> GDPVEDIIHDALSSTVRRAITSGQDVNTAAGTAPSSHRLETGRVPALQAAETGATSNATDENMIETRCVMNRNGVLEATISHFFSRSGLVGVVNLTDGGTDTTGYAVWDIDIMGFVQLRRKCEMFTYMRFNAEFTFVTTTENGEARPFMLQYMYVPPGAPKPTGRDAFQWQTATNPSVFVKLTDPPAQVSVPFMSPASAYQWFYDGYPTFGQHPETSNTTYGQCPNNMMGTFAVRVVS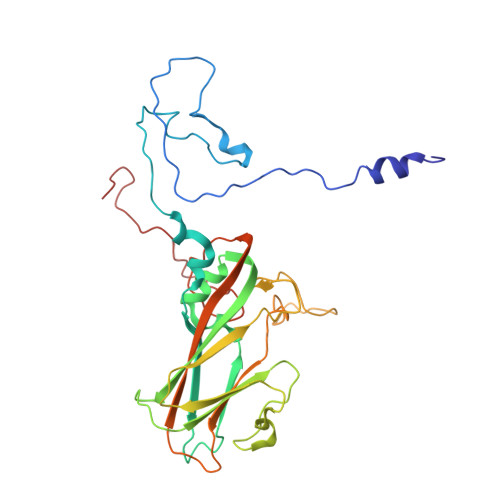RVASQLKLQTRVYMKLKHVRAWIPRPIRSQPYLLKNFPNYDSSKITYSARDRASIKQANM> MGSSHHHHHHSSGLVPRGSHSDEVDAHMTTNTVSRKVAWLRVVTLAVAAFIFNTTEFVPVGLLSDIAQSFHMQTAQVGIMLTIYAWVVALMSLPFMLMTSQVERRKLLICLFVVFIASHVLSFLSWSFTVLVISRIGVAFAHAIFWSITASLAIRMAPAGKRAQALSLIATGTALAMVLGLPLGRIVGQYFGWRMTFFAIGIGALITLLCLIKLLPLLPSEHSGSLKSLPLLFRRPALMS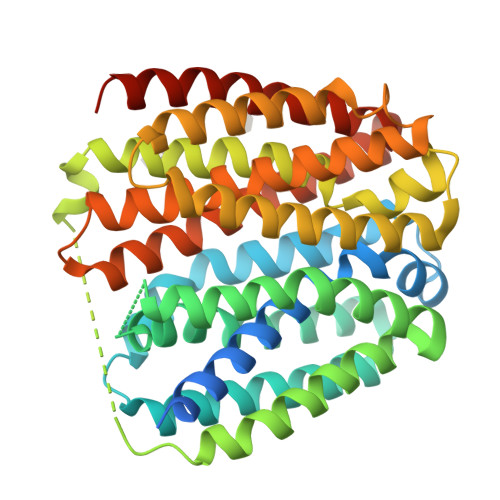IYLLTVVVVTAHYTAYSYIEPFVQNIAGFSANFATALLLLLGGAGIIGSVIFGKLGNQYASALVSTAIALLLVCLALLLPAANSEIHLGVLSIFWGIAMMIIGLGMQVKVLALAPDATDVAMALFSGIFNIGIGAGALVGNQVSLHWSMSMIGYVGAVPAFAALIWSIIIFRRWPVTLEEQTQ> DNYADLSDTELTTLLRRYNIPHGPVV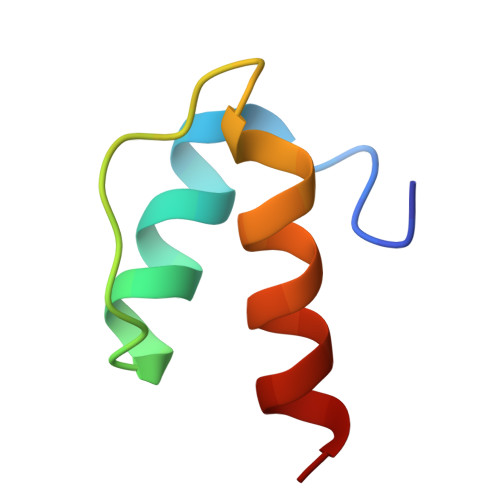GSTRRLYEKKIFEYEIQ> GSWFFKNLSRKDAERQLLAPGNTHGSFLIRESESTAGSFSLSVRDFDQNQGEVVKHYKIRNLDNGGFYISPRITF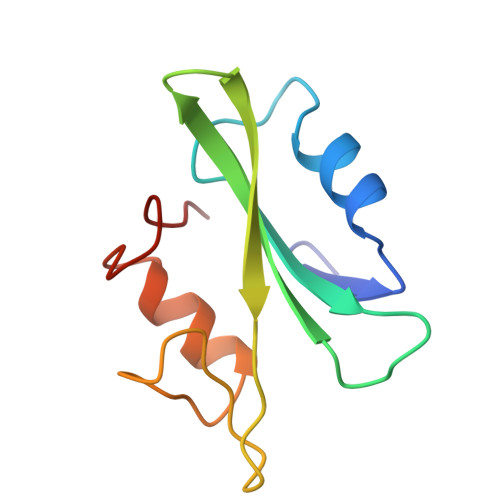PGLHELVRHYTNASDGLCTRLSR> MGGSGSRLSKELLAEYQDLTFLTKQEILLAHRRFCELLPQEQRSVESSLRAQVPFEQILSLPELKANPFKERICRVFSTSP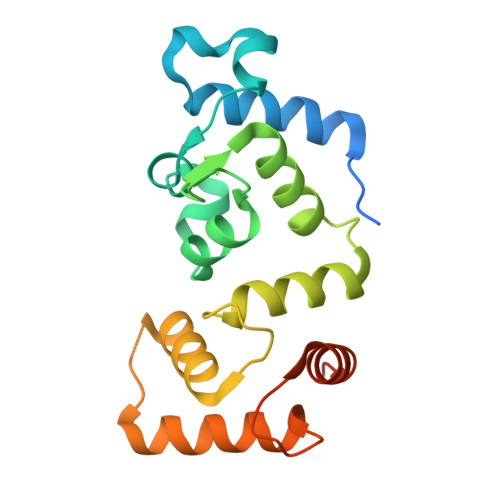AKDSLSFEDFLDLLSVFSDTATPDIKSHYAFRIFDFDDDGTLNREDLSRLVNCLTGEGEDTRLSASEMKQLIDNILEESDIDRDGTINLSEFQHVISRSPDFASSFKIVL>[2x]MLAGIYLKVKGKTQGEIKGSVVQEGHDGKIHILAFKNDYDMPARLQEGLTPAAAARGTITLTKEMDRSSPQFLQALGKR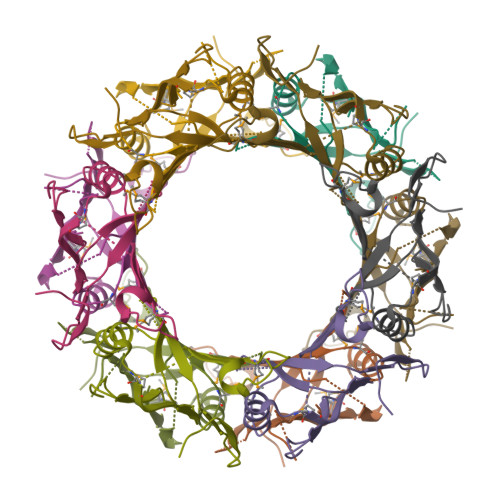EMMEEFEITIHRPKTDTTGGDLTELLFTYKFEKVLITHMDQYSPTPHKDDSNGIKEGLLGYIEEIKFTYSGYSLEHAESGIAGAANWTNG>[2x]MHHHHHHMTYENLDAKLINALLGDGRASLRSLAEELDVSVTTVSNHLRDLEDEGVIEGYTPRVNYDALGYDVTAVIQLKVEGSALPEITERLRAEKQMISVYEVTGD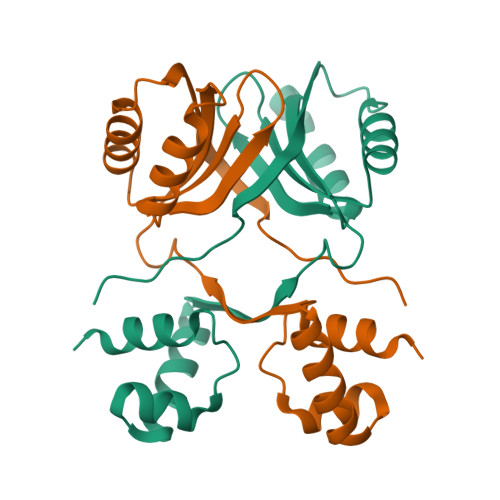YDIIAIGKFRDTDGMNTQIKKLLTDTDIRESNTSVVLNAVTENEQFALDVDE>[2x]MDALQ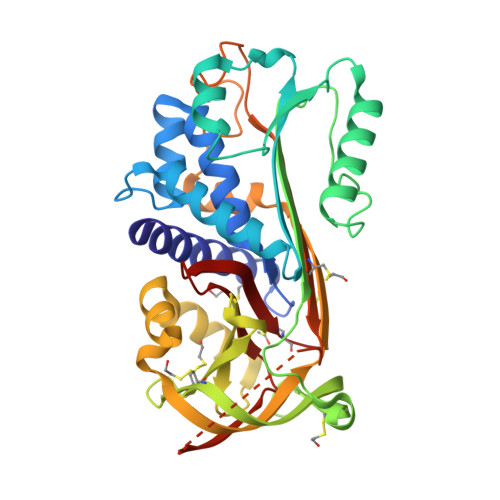LANSAFAVDLFKQLCEKEPLGNVLFSPICLSTSLSLAQVGAKGDTANEIGQVLHFENVKDVPFGFQTVTSDVNKLSSFYSLKLIKRLYVDKSLNLSTEFISSTKRPYAKELETVDFKDKLEETKGQINNSIKDLTDGHFENILADNSVNDQTKILVVNAAYFVGKWMKKFPESETKECPFRLNKTDTKPVQMMNMEATFCMGNIDSINCKIIELPFQNKHLSMFILLPKDVEDESTGLEKIEKQLNSESLSQWTNPSTMANAKVKLSIPKFKVEKMIDPKACLENLGLKHIFSEDTSDFSGMSETKGVALSNVIHKVCLEITEDGGDSIEVPGARILQHKDELNADHPFIYIIRHNKTRNIIFFGKFCSP>MDIISVALKRHSTKAFDASKKLTPEQAEQIKTLLQYSPSSTNSQPWHFIVASTEEGKARVAKSAAGNYVFNERKMLDASHVVVFCAKTAMDDVWLKLVVDQEDADGRFATPEAKAANDKGRKFFADMHRKDLHDDAEWMAKQVYLNVGN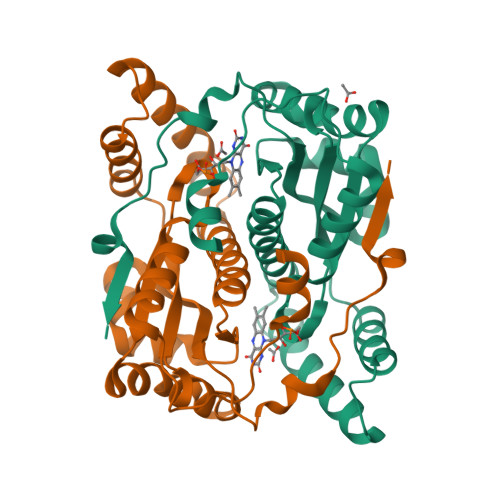FLLGVAALGLDAVPIEGFDAAILDAEFGLKEKGYTSLVVVPVGHHSVEDFNATLPKSRLPQNITLTEV[2x]>[35x]HEFAELFYRTYIVTPDQAGFQLSIRRNLVWEGWTGEGLSGEKQEISKRNILQGLLDYTTLETNSTELIPVIQSGENDEQFIDPSVLPAQTVKQGKDTFDTNFLKFSENGEGFNLLMLAQTPSRLKKGSMTFTDSLDSRIALKQLLISVTKGGTTELFALDVNRDQYAAYTATREYNFRLMQLKFHTSLGLGEESTTVAGAESALLKDLFDLGYRIELDVKVDGEMNVENGNGDTSLRALRLARVFDKEGKEIALTDSRVSAALSGLTVTGVGYSLEARLTNINQLEMGLLIDSDVQKQGFMIPTLPPLVIVKPAMVEDDKTYPRLEALTTAYRIQQMRNNAVTTLLNRADTLKSYLGVGVPHPIESNLGLEGVGQYYVRPYYNEATIDVLNDLNNLTSAAKQTDIQGLIVSKINEMVYTADQLTGYTAALEAAFSGRSPKPHVAIGTDMRLPQYIQINGDDRTVGIGYDYTIARISDLRMKDKIVMTFILPNESEPHPLQHGVLGFIPEYLVDFNMIRNQRIGREIRLTPRYRYFNFLPIMLVINVINLEEAIAQRTALDVNETQVTPAS

The Klebsiella jumbo myophage ϕKp24 displays an unusually complex arrangement of tail fibers interacting with a host cell. We observe the tail fibers are branched and rearranged dramatically upon cell surface attachment. This complex configuration involves fourteen putative tail fibers with depolymerase activity that provide ϕKp24 with the ability to infect a broad panel of capsular polysaccharide (CPS) types of Klebsiella pneumoniae. In this study, we combine cryo-electron microscopy methods, protein structure prediction methods, molecular simulations, microbiological and machine learning approaches to explore the capsid, tail, and tail fibers of ϕKp24. We determine the structure of the capsid and tail at 4.1 Å and 3.0 Å resolution.

Each pentamer consists of five MCP monomers. In comparison with a gp372 in a hexamer, the N-terminal in the pentamer’s gp372 shows a different folding direction. In addition, gp372 in a pentamer changes the relative orientation of the triangular body and the hand compared to the MCP in a hexagon, which makes gp372 more curved in a pentamer. Overall, the MCP interaction regions in a pentamer are similar to those seen in the hexamer. However, the increased curvature of the pentamer alters the relative orientation between the triangular body and hand regions, leading to differential stabilizing contacts. Specifically, in the pentamer MCP, residues R501 and R583 in the triangular body interact with residues D448 and E442, respectively, in the triangular body of the clockwise neighbor. The interactions with the clockwise hand region are reduced overall, involving residues K380 and R558 interacting with residues E220 and D163, respectively. In contrast to the hexamer arrangement, the C-terminal loops in the pentamer do not appear to form a large, well-defined pore in the density map. Instead, they are disordered, perhaps owing to this different arrangement to the reduced space and greater steric hindrance between the MCPs in this region. Nevertheless, we do observe a small opening at the center of the pentamer that may be capable of solvent transport.>MAHHHHHHSSGLEVLFQGPMALYDLTLAELEERLAADGVPRYRARQIFHWAYRQLAVDYDAMTVLPKTLRADLATRLPLTPLTPVREVQTDDGETIKTLFRTVDGQHIETVLMFYPDRTTVCVSCQVGCAVGCSFCATGMMGLTRNLTAGEMVAQVVAAARRAREAGRTLTNIVMMGMGEPFQNYEATMRMVRILHEEEGMNFGARRITVSTSGLVPFIDRLAREPFQVKLAVSLHAPNDDLRSSLVPLNRRYPIGELIAACRRYVGETGRRVTFEYVLIDGVNDSDANAEELARLLRGLLCHVNL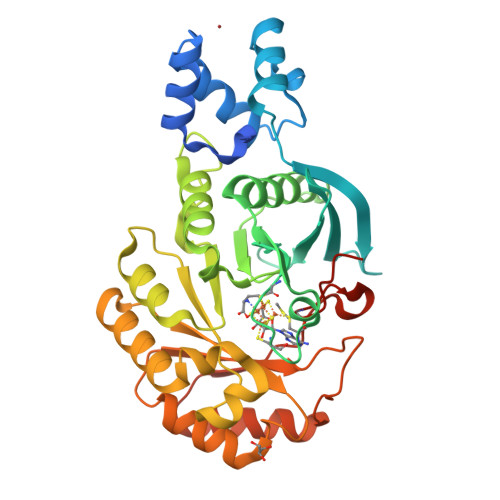IPLNPTPAAPFGRPSVERINRFEQILRARGIPATVRYSRGVDISAACGQLRAEYEAVAGA[2x]> MLSSKYSKRIAWMKTTICDSLQLKDMIVEESFQYEKNKNLLEQFLSGEGLNKIFAYYQVQEQAQNDDIKDTGAQDPVLFFTTGDLEKIQDKAVWFLRITNPADDKKKASQQDGNDNDIIFGEITPNTVPMLNALMESVYSRQIDHIITEKIQFWGVAEEEQVLEFQQHSNKFSSEVREAINLMSPGTEHFKLDYEAISGLSESEKMQHYEMKFNEWINLISSQLNDDSEVRKDEKDAGPATELIYWRSRMQKITNWSEQLKSKDFQIVKASLQRHKNHDNQRPRGDESLSKLMMEYNRLDLLLTDKLNEAKDNVKYLTTLEKFIEPLYNGTPQQIIDTLPALMNAIKMIHTIARFYNTTDKMTGLFIKITNQMIKNCKDRILNKKDNGDNPSLYKMIWEQDPAELIEVLGSCIKLYCEYKKCYNDTKEKVADMPKGKTFDFSDAQIFGKFDTFVRRLQKLIEIFSNIQQFNALAKHNLEGMDVLTNKFKKIIDDFKKKGHNLLDTANNKFDRDWVEFNVEISHLDGELQNFIDNNFNRFRNIEYSLKLLHKFQSTIKRDSLKHNLTSRYNAILHNYATELDTIQRVFQDQKSNPPLVRNMPPEAGKIIWARHLFQKITGPINIFPENVINSTEIRRYYGSYNTLGKQLTIYEMWFYQDWVNKIEQSKAALQATLIVRHDENKKLYVNFDLEIMQLIREAKCLDRQGIEIPESARIILLQEDKFKTYYNELLYALKEYERINSKIKPICKNLLLPHIEDLDLKLRPGMVTLTWTSMNIESYLYYVHQGLKKLEQLIINVNDIIENRIENNLKTVSKVVLVHLPQDTKPLSLDSFVQLQEEYINSKTDFLTSKNVEVERAVDDLLQTIMLYPLDPHVDPVLPEETKRIKRYYFWYFYQALLNSTQNSLNAMKYRVCGKKIPGANTLQNLKPFFQVEVQLNGDKVTLNPSLQEIQKSINRAATAVLRCSKHLYNWDQQNKDSTDKATFYDMIACDKEIVKVILLLTGSIQGTKNKVNEFLSGFTKFEWLCKESIQESIKKFSKNGPTLQNYEDQLKKFSQIEEEIEKIVPTYKIGAMELMTHNICTSLSTWAKEWKLQYSQDLHKRARQLLDSLTEQTKMLSTKLSKPVKDIDSLGYVMETLEQIRKEQAEIDMKFNPVQEMYSLLDNYLPGGITDKDEMDARSLLRRNWDILIQQAEIKGKEYQHKQAIYLKELKQSIKDFTNQVSIFRRDYEKNGPMVEGISPAEAMERLRRFEDEYDVKYQMYKINARGENLFGLQNQKYPELEKTDAEIKNLNKLYNLYDSVIKNIQQFKEKSWQDVSKDDLAKMEEDAGKYGEQCSRLPKDLKEWQAYRDLKNYIDSLREQLPLIISLKKPSIMPRHWEKIKEITNTKLNYENPDQFYIEEIMGAKLLDFREDIEDITESADKQLKIRTGLDEINLYWNDMQFQFGIWGKRDVPCMLNGLIVGTILERLEEDQLQLSTFNSQRHVTPFKAEVENLIRTFSDVNDTLDMWVKVQKLWTSLEPVFTGGDIARQMPLQAKQFQGIDKNWMKIMEKAVETKKVIPCCQNDMLKDFLPDLNRKLEDCQKMLEAYLEGKRKKFPRFYFVSNPTLLKILSQGSEPTSIQEDFEKLFDAITKVTFESAKDKKNPALKQITQIQQVIGRNEENISLTGYYVKCEGNIEDWLKKLEQNMQQTLKDIASAAAQQVFQVGLKEFVSSQASQIALLGLQILWTSKVNEGLERLSRNERNAMDIKRNEIKEHMNILSSMCLEDLNGAVERTKVETLVTIQVHQKDISMDLKCKDVNDFEWQKQTRIAWKTDIDECIISITDWDSPYSYEFLGAKERLCITPLTDRCYITLAQAMSMYYGGAPAGPAGTGKTETVKDLGRTLGVFVVVTNCSDQHRYRDMAKIFKGLVQSGLWGCFDEFNRIDLEVLSVVAMQVESITTARKQHMKKFMFPEEEIEIELIPTVSYFITMNPGYAGRQELPENLKVLFRGVSMMVPDREIIIKVKLASVGYLQIDLLAKKFNVLYRLCEEQLSKQRHYDFGLRNILSVLRTAGNTKRQEIKSDEEMLLMRSLRDMNLSKLVADDIPLFNGLLADIFPKLKEVPKKLYPDVEKKIPEEINAESYLINTPSFQLKIIQLYETCLVRHGFMLVGPTGSGKSTIMKILTEVLTKLGSPHKIVIMNPKAITAEQMYGVKSEISDDWIPGVFSTIWAKSNNRALKHTTWITCDGPVDAIWIENLNTVLDDNKILTLANGERIAMTENCKVVFEVENLNNASPATVSRCGQVYVSPTDLGYEAVIEGWIRNRKASGRAEESDKLGNILRKYLINMRFIELQSKECKEPMMDTSPVISVINILNLLTGCLQYFVQTQRTLSEQEYEKFIVYSMAWAIGGIYEAQDRVRFHELLLAKNAPIPQKGKENETVFDYYVSQDYLDWKICSPEEWVPPQSLQFSQLLLPTLDSFRAEMLLNFILTQPKSHTCSNSALLIGGSGTAKTSSVLLYCNKFDPQKMLFKRTNFSSATSPFMFQSTIEAECDFKVGKEFAPPGNKMMTIFIDDMSMPFVNKWGDQITLELVRQLIETGGFYMLDKTQRGNQRKMKNLQYIGAMNHPGGGRNDIPNRLKRQFFIFNMILPLSIEGIYGPIIKHMFKQKYFSDSTYKVIESLTSATIALWNKVKSTMLPTPAKFHYVFNMRELSRIFKGILTCKKDTINDAPKSMKIKPELFLVGLWRHEAERVLADKLVNNKDKDTVMGYIQEVSLESFSQIENEILEKYSSEKTFLFCDFLRPDVINEDGIIEEEAPKIYEAIDSLTELRKRCNFLLSFYNDRNPSKKMPLVLFDDALKHLLRISRIIRQPRSSGLLVGVGGSGKQSLTRLAGFIGKNLIQQIIVTKTYSDKDLKEDIKKGFDDAGHLGKQVTFLMTDSEVKKEEFLEYINMVLSTGEIPNLLAKDEREVWLGDISQAYCKEKNLGNIDPPQSELWTYFVDRVRDNFHIMLCFSPVGQKFRERARKFPALFNECTIDWFLPWPEEALVSVAETFIKNFDKLDTKEETKQELMKHMGNVHLMVNEICDEYYQKMRRQVYVTPKSFLSYLNSYKTLYIEKYDELDQQEESFKIGLNKIQEATITINQMEISLKEEEIQLNEATEKTNQLLANLDKESKKANQKGEEVAATNKQCEIQAEQISKEKEEAERELEAALPALRRAQEAVDSIESKDIVELKANKKPLDIIKYIMDAVLVFFKARLIPIQIEERVFNKKEGKAVLFLKESYDESGIQTLGDMNFMKKLKEFEKDSINEETIELLEPYLNQSEDWFNDTFATKASKAAAGILKWAFAIYEYHQKSKIVKPKRIQVAIAEGRQAIALKELEKAREDLAQIQAYIKNLKDVYTKQMEEKNELEMKAAKTKKKINTARTLITSLSGEKDRWGKGAQDISDQKRKLVGNVSLSTAFISYCGPFNAEYRNKLAQQRFVVDMKKRGVPVTPGLELTSFLIDDATIGEWNLQGLPKDDLSIQNGIMVTNSARYPLFIDPQGQGQNWIRNKLSASIIPERCITTLSHPKFKDMFLKYCMESGLTLIVENIENEVDPMMDPVLERQIIVKGKTQFVNVAGTEMELSKEFKLFMTCRLANPSFSPELSAKTTIIDFTVTQSGLEQQLLGKVISKEQKALEDSLNQLLADVNQNQKDLQRLDKNLLERLINSQGNLLDDTELMDVLNNTKTQAKEVAAKLIDAEIKTKEINEKREQYRPVAIRGSAIYFTMIEVSLVNWMYNSSLEQFLKLFIESIDLSEKAQLPSNRVKNIISFLTFHVYRYVNRGLFEKDKITFILMMAFKILTTAGTISSGDVSLFLKSGDALDIKSERQKQISYLEDNQWLNILALSKHTFSGQTLPFFKELPDLISRSENQWRNWIDKNDPENFPIPDFAESINQEKEIGSFISLCLVRSLRNDRTLIATQNFISNVLGKEFTDPISYPIEGIWQESSNMDPVLFLLSAGADPTSSIDELAKKKKKFPCEKVSMGEGQERVARQVIMKGFVEGGWVILQNCHLGLKFMEEIETLVSPINQIHEDFRLWITCEQHPKFPLGLLQKTLKVTNEPPKGLKAGLYKTFTTIITQEFIDKVDHSNWRSLIFTICFLHSIVIERKKFGPLGWCVPYEYNYSDLEASLLYIEKYLTNLMSTPQPNSHNLPISMNVVRYMICEVQYGGRITDDLDRELFITYGETYLKDGIFGNDYFFYDIMVDGSGQKFKYRIPQNPSAELIKYQEYIAKVPTVDNPEVFGLHSNADLTFRLKESKEMINTVMETRPKDSSVGGGKTREEIVQDKAKDMLKNLPPDYNDVEVRELVSKLGGPNPKTSTERGMTVPLNIFLYQEVTRMQRVIGLVRKTLQDTILAIDGQIIMTPEILEAINAIYDAKVPNSWLYDPSGAEISWLLPNLGSWSTSLSDRNKQLNDWLRSGQRPILFWLTGFFNPQGFLTGMKQEVTRNHKKKDGKGGEAWSLDDVVYSTTVKEREKEKDIEQPPAEGVYIKGLYLEGCKWSKNGLDDSDPKKIFADLPILHVSAINKKKTNEQDRMSNTYLCPVYKYPKRTDKYLIFRVGLPCEGSNNPSHWKLRGVALLCSTE;> MGDHSQKDSPEDFIINRLSQALGIQKEKIKKSLETQQDDKGEVTNKDEFQGFIQQDNSTNILWVSGQSEKCTFYYGQLPPIDKFKKKGIAVIKLGLHKLTNENVAKDVVVVEITNNLLEHLNSVFNEIMSPVMQNPLNQQGWTDLVAKDLMEKFNNYVAQVYVLLGQIKGKTMLPLPSHKLTSSDTTPDKDKAHVFEGSIITWTKQIKNVLKLEPEQLLKYGNDPGPLAEIEFWQNKRDNLNLIDSQLKSVEVQNILHFLDNNKSTYTTPFTKLQAEVKKARLEANENYRYLFTLKDLFSKLQESQPSDFPTLYELFIPIMHTILLIYNKSKTYNQPPRLVVLIREICNAIISNAQAFVDKDTIFSLIDSKETTEACDKLQVTLDVCSKFKDAYFEYKAKAGGNWKLTSNALFVRLDSFLERCQDILHLTNTIVQFNKLEKIELGGTKGKTLTESIAQIFKEFEEAVQAFTSVSYDIMNIAEKKFDDDFYEFRSKIKELERRLASVITQGFDDYDTIYGRFKLLDNFEGLLTRPIIADELEKKHIVLLEMYKQDLKQVQSIFLEGKQFVDSMHENAPLFLNMPPIAGALTWCKSLRDRIQEPIEKLAQLGQGITEREEYKDVQKLYTSITKSIKDYEDQKILSWEKEVEDSSQDKLKQTLLCKDENDLIKVNFDPSLVRLLKEVKYFLLLRLEVPTTAKDIYTKAETYRTQIVALDMIVDNYNHIKTCLLPVEEPLVKKKIQDMEEEVKPGIEEIRWKSTNIDQFISKSKSIVDQLFETVNKMKDSLQKIHKSLANFNVKIIERKNRPMSPDDYDQFLKAIFSNKLTIVKDNGNQIQKLVKEVLDAVKADKKQNSWKNYNDYVNVIVIEGISTAIQTALLHLNEQINPVFIKRNDISPLFDIRLELGQSGIQFDPEIGESSNQLTVRNTIRNWINDFFNIAGTIQRLDTTMPGDFLQEIRSFFEIKQCLAMITQNLEWIENECNQFRARFDTYSYLWTEDEQISFNRFLDENEPKDEDGKGGDDDEGENTEKQNPLLKGCRAKIPNLDLFDEKITHLKAIQQEISRIKTPEDISWLRINLQPMKTALDARVTRWIRVYTDFLVNQFRTTQKNLLDFIEKTKDGIKKNPADHENLHDKKLLMSVMKVISDVKDVEPRREGIITRMKEMVTKLKKHNVPITEKGTDDPLQQIDNANSNFIEIYGRVFKVKADIIPLQAEETQNIKRDLDIFMKEVESFRKEFMQKLPFDYTESMGYENINNAYDTIMVYYHKLTAIEGRALEYNNLEKLFELQKSNYKQLKDCMNDLKNLKTMWDAIALIHFQYNDWKTKPWRQIKADILLDTNKTLGTQIKNLPKEIRNFKGYNVIVEKVKNMGTVLPLVSALHSEFMEDRHWSQLKQITGTVFDHNSLSFYFEDILALNLYKYENTVNEIVDVAQKEAKIEKKLKNIEQWWSKQVFEFTEYKETKTFASLDNMMEVLDQHSLDLMGMKSQGKYVEFFYDRVEDWREKLGRVDVVVNEWLKVQKNWKILYNIFLLSEDIRMQLPEDTKVFEGVDKEFKDMMSEVSANPSVVEACTIERRDVLVGWSQAIKKCEKALNDYLEQKKKSFPRFYFLSNQSLLTILSNGQNAPKVCEYLGDCFDGLKTLTFEPPANPAETSKVGIGMISKDDEKVPFSSKFICEGAVEHWLLNLEFRMRETLQEILEGAKNTADLWDSGDKPREEWVEGYNAQIALLTTTIVWTEDVGRAFEDLAGGSETAMKECQKLIEVRLENLIKKVRGDLHILERWKIINIITIDVHSRDVVEKFVIQKVSEAESFAWLSQLKFYWENKPDSDMHLRQTLRFPWEKDKNKNKCIIRIVDWFRFYSYEYIGNAIRLVITPLTDRCYITLTQALNLTMGGAPAGPAGTGKTETTKDLGRAIGIPVMVFNCSDQMNKDSMAQIFMGLSQSGAWGCFDEFNRISIEVLSVVSTQVKCVLDALKEKKTKFSFVEEGEIQLQDTVGFFITMNPGYAGRTELPENLKALFRSCAMVVPDLALICENMLMSEGFTMARVLSRKFVSLYMLSRELLSKQKHYDWGLRAVKSVLRQAGKLKRGDPDMPEDPLLMRALRDFNMPKIVTDDKVIFRRLIGDLFPKLDPPTKQNPELKKIVQDTTKKDMGLVAEELFVTKVVQLAEILEVRHCCFVIGPPGSGKTCVWKTLIKSYINSGEDAEYDTLNPKAVTSDELFGAYTKTKEWKNGVIAVIMKNQVKNEEKYKATHMHKWSVLDGDIDPEWIESLNTVMDDNKVLTLVSNDRIFLTPQMRLIFEISNLRNATPATVSRAGVLFINETDIGWMPYMNSWLERSQINILKQQKEMANMPEYPVIDDVAKSVFYRCFQSYFEQNIDVHDKNRVRHICPMVDIAMIQTICTILDALLIQHLPKLKQMKEEDEKQALEAFFIFAGLWAIGGPVGGGQDDSKDMKEFNTVWKGAAKVKFPEQGLCYDYYYDINENKWNTWKVEDYLPNDQPLFSKIYVATIHTTRLRYMIDIHLQRRKPILFIGSAGTGKTAVVRDYLNSTRPEQVSHKTINFSSFTDSLALQKNIESMVEKKNGRNYGSATNKVLICFIDDFNMPYVDKYGTQSPIQLLRLILDYGSIFNREQLEERKFLQDLLFFGCLNQKSGSFTVDLRLQRNFSVFSMYTPSSDVIKTIFGSILNAHLSTIDDKAQKMAFKLVEATYFTFDKILKNTTAFAPSAKRFHYQFNFRELARVCEGICRTTPGQYSGGDQGKLVRLWAHEMKRTFEDRFIANEHVEFFRRYLTEAISKCIGEFPETENPIAEPLIFTGFVAAHQGLDQQYTQCTIPVLKRVLDDKLEEYNEVKAQMNLVLFQQAMEHVSRICRILDMPGNNALLVGVGGSGKQSLCRLSTFINGFEIDQLVVTASFTINDLRNNLQEIYKKIAKPNSIARVFMITDSQIKEEQFLIPINDMLNSGWIFDLFPKEDMDSLVSGVRNEAKGEGVDVNNLTALTSYFLDKIRKNLKVVLCFSPVGDTMRIRSRKFPGIINNTSIDWFHPWPHEALIDVAFRFLEEIEFPTEEIRQSISLNMAKVHSSIDTANEKFLKLERRYNYTTPKSFLELIDFYKKLLTEKRETIQRQIQRYEMGLNILAETQNKVQGLQEELKVKMVEVNKQREETDILIEKVGKESALAEEEQTIANAEEEKTNVAAAEAEKISKEATEALAEALPALRSAEAAVDCLKKPHVTEMKNLGSPPAGVIVTARVVLILFNQGITLNDPDEKVWKKAVTFMNNPQAFIDKVKSFDGENIEPNIIEQSNKIIQDPSKKFNEKDMAGQSYAASKLCAWAVNIVTFNKIFKQVKPLQDAQKQANEILEEKKKELAIVKQRVAELNARVNSLKRQLEEAEARKMIVEQDAARCQSRLSAAENLVNGLAGENKRWTQNVKFLKENIKSMIGDSLLASAFVSYIGAFSAKLRLELWKNTWLPDIIEKGIPITEGIEPLKILTTEAIKSKWKNEGLPADPMSLENAAIITACARWPLIIDPQLQGSTWIRGKQGENLTTISLSQPKWLGALTSSISSGRAVLIEGIQQEIDATLDPLLQRAVKKNGNQLQLEIGGDPIDYDPNFKLFLMTKLINPHFRPEIAAQCTIINFIVTESGLEEQFIAMVVNIEKNELEMAKQDLVKKQNEYAVTLDKLESDLLQSLSEADPATILDNTELIQNLDKTKKTTIEITEQQQKAKVTEAEINIQREHYRVVAAEGSMLYFLVISLSVMDHMYQYSLESFITFFFKAINRTTVRDENRIPTLILNIRQTIYQWISRGLFEKHKLIFLTLIVFRLMQKKIIDVAYEVAEMDFLIKCPARPGVENTLDWLPNISWDQIQGLINLEEFRNFAHQLEKEAPNRFKDWYNELQPEDQKLPLDWKRLDSMPFKKLLVLRCLRPDRMTISLNNFIRAVLPQGDAFVEMDQKLAFSEILESVINEDSESTIPIFFILSPGSDPVKEVEKIAKKKRIEPGKNFFNIALGQGQDEIARRRIEEGNKEGHWVMLQNIHLMPTWLIELEKILDSYSGEAGGGNSEFRLFLSAEPSTGIPIGILDRSIKLTNEPPAGLKANMKRAWTYFSKEEIEDKDPKIKSILFALCFFHSTLIERRRFGPKGWNMSYPFNMGDLRDSYLVMNRYMEQNQGGKVPFNDLIYIFGEIMYGGHIVDDWDRRLCNSYLFNTMHEQLFDELELFPYIEGKGLSFKVPGQNPYEKYIEHIETSLKQETPLAYGLHPNAEIGFRTDQCKTLFNTLLELMPKEQSRDEKSSDIKSSNEMASDLIKQLLEDSELKNKIFNMEEIKNKIDAENKGPYQNVFLQEIEYMNALLSEIVKDLEEIGQGLSGLLTVSENMEMIIESIALSRVPASWQKLAYPSKRGLQSWLANLFQRIEQLNIFRDDPYSIPRVVMISRFFNPQSFLTAIMQVISRAKAYELNKLYIQTEITKRSIEEIEGAAKEGAYVYGFILEGARWDYQLGQLEESKPKEMFSVLPVTYCKAIPLPPEGKEDKSLYQCPVYKTEDRGNTYVFTAQLKTRFPPRKWILAGVAIIMDVEGVSDEVKKDKK;> MPQPLVWTQLKQTGTTQPTARSGHTIITVGKTHIMFGGLDNDKNNYKDGKIAPNNQVFTLKLTQNNCEWRQIACQGDVPLPRCYHASCAISADKMLVFGGSYTSNLRFNDTYILKTTSYQWSKPANQISGGEPKNAESKIGAPQPRYGHSATFFEGKVYIFGGHGGINYQRLAFNDLYVLETENFEWTRLEPKGNPPDPRGGHSAAMMANKPQLMIFGGWSFTSQYSNIMIYDIEKDEWVDPEIAHEIPKWNLSGIMAPSIPSWKYFIFGGSVGSFEEGGNRTNSRFVDDSFVLDIDTLSWSSINLEADETSKAVCKPRPRESASIFYDSGESRAIVFGGWANNWLNDLWALNVSTITGPPYAIFSIKPALGPLTGKTKVLIEGDGFKDTQNISVKFSGGKLEKEVNGTFVNEKEISCETPTFDYPRSVEVTVCMNKGDYTITKSAFTYYLNTKADKTIAYGPGLLTENLIGVQTTIVIQARNKNDQNRESGSDEFVVTIRNPAKIKKEEEVKEGDKANTKNTIKEDEEEEGEDEEENKKKKEAEKAAAEKAAAEKAAEEEQGEAVDPSLVPFNIVDNDDGSYFIQFTSEEEAVLEIDIKFKDENNELHSIRGNPFRCGFVKGSKPNNNDLTGSAVMNYISKQLKDIQEFIENTKENIEIRNKNIRENVSELINVMINLEKVRVKNDDDVLTLDTVEEMLNFLKKKDFGKDSDIKKCKKLQEEWKNLAKMAQAVKKDIQNPVKTESDKTKENIKKFEEITLKEYANSLKKESFFIYKTGVSESFKRIG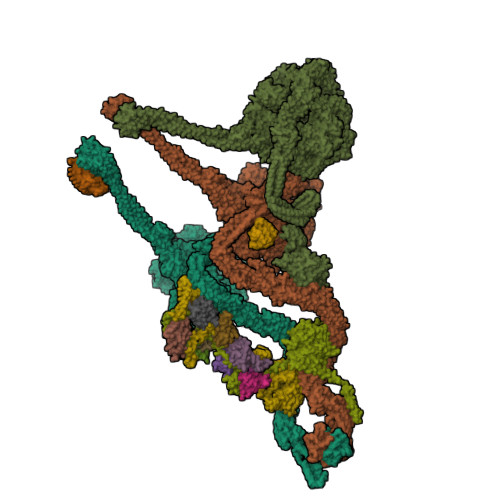EVKQKVDEFEVQLNQYEDFARMFEFPDAVIGSKKLMEQIRTDVSSVEKLWVRIEISEKTMDEYKKMKWGSINSMDMEDEIKKLRKALTDLRGIDKRSNAFIGITEELKKWATFLPLLGELKDPSMNSEDGRHWKKLKDLVKKEFDVSQELMLEIIWDLKLFDYKDGIEEITDQAKQELKMEKALKKIIDFWRDIEFELVQHKNTDIHTLKMSEENFETLEDHQLQINNMLLSKYVAYFEKEVEKWKYDLGSVYDVVQLLLEVQKTWSFLENLFIQSEEVKRELPNESAQFVGIDKDMKEIMQKGCDIKNCLKFCTIEGMLKRLENIQAQLKVCEKALNEFLDSKRRAFPRFYFVSVNDLLDILSNGNSPAKINRHMSKIFQAIDNLQLKEDSSGGRPTALKMISCVGTEEVDFSSPRLLQGKVESYLKDVIDTMIGTLKSVANSSFKNFQSMTRKEWLKSDPSQITLLVNNIIWSKAVEDCFLKLQSGDINAMKLFLDESIKQLTELIGMVQGDLSKPLRQKIMCLITIDTHSRDVVHRLINEHVRKAEEFQWQSQLKFYWVDNDAKIKIADARFVYNYEYLGNGPRLVITPLTDRIYVTATQALHLKMGCAPAGPAGTGKTETTKDLANALAKACYVFNCSSEMNYESMGNIYKGLASSGCWGCFDEFNRLLPEVLSVCSVQFKAVTDAIKQNVERFIIEGDEISLDPTCGVFITMNPGYLGRAELPEGLKALFRPITVVVPDLELICENMLMAEGFIEAKILAKKFVTLYMLCRDLLSKQLHYDWGLRAIKSVLVVAGGFKRSEPEIAEQALLMRALRDFNIPKIAFQDLYVFHGLLGDLFPGINIKPKKDLDFEKIITDVCIENKLDPDPEFVLKVVQLSELLAIRHCVFVMGPPGAGKSTTWKILAKAQDKTNKKTTLIDIDPKVVSTKDFYGYNLPSKEWKDGLFSKMLRSLAEQPDTNPKWICLDGDLDANWIESMNSVMDDNKILTLANNERIPLKPHMRALFEIRDLRFATPATVSRAGILYISDEVGYQWRSYVKSWIKQEFSQDQEMSKNLDTLFGKYVPDTLDHIKKHCRFLVPVSPISQVISICKSLQTLLKGDVKNLEYLFVYALIWAIGGALAEKDSIDYRKDFSTWWKGAWKTAVKFPSKGTIFDYYVDQSGDSSKFVEWSKRLENKEFDPQVETMGNITVNTIETLATTEFIKSYLMVKHPSLLIGNSGCGKTQLAKGILKEIVQAKPENYAYQLINFNYYTDSTYLQGQIEQTLEKKAGRQYGPPGKVQLIYFIDDLNMPQLDAYDTQTAIALLRQLADYGHFYDVSKLALKDIINTQVLAAMNPSAGSFFVNPRYQRHFWTISIPFPDNESLSLIYITFLNGHLKRFKSTIQEYSNIIVRASLMLHQAVTQNFRKTAINFHYEFNLRHMSNVFQGLLLSDPNKFTEPDKLIKLWIHECERTYGDRLVSTDNLKTYKENIFDIVKKSFSKFNFSRYFGNNPENLIYCNFIAGINSDRFYDQMPNNEMEKHISEALKEYNDNNAFMGLVLFEDAMKHVCRICRIVLPSSGHALLVGVGGSGKQSLSKLASFIMGYTTFSITISATYSMVDLRNDLQQLYFKCGPKEEGILFLFTEGQITNERFLVYINDLLSSGEIAELYTLDEKEAMINQVRAKVKGEGKPDTRENCWNWFIDQVKKNLHMAICFSPVGDMRRRARQFPALVNCTVIDWFQPWPYEALFNVAKSFLEPVDLGDDKVREAVVKFMPFSFTLVNDLGLKLLEQERRYAYTTPKSFLELISLFTNMLAQKRESLERNKERYETGLVKLKETAEQVAIIEVEVKEKQVEAEAKKKEADAFAEVVGREKDKVEKENSKATIEADKCGLIKQNVEAQKSSTQQDLDAAQPLVEQAKSALNSISKKDFQQAKSFASPPAGVPEVFAATIYLLAGYFNEAIEIDKNKKPKDVSWKSSLKLMKSPEEFMEKLLNFKDVVDANQVPAANVNIVKNQYLNMPSFTPEQMASKSAAAKGICSWVVNIVKYYDVIQDVEPKRKALKEATEQLEEATVKLNEVEEVVRKLNEELNKLKAENDKAIAERNAAISEAERCARRLNLAQRLVTALSSENERWGKSIIQLEDQLKLMVGDVLVASSFVSYSGPFNKKFRNIMINQNFMKFMKEHTIPMSPDPNPIKILTDESTIALWNKQKLPSDSVSIENGTILTNSARYPLMIDPQLQGITWIREKEKANNLKILRLGSKNINRDLELSIENGYSAIIENMNERIDAILMPIIARSFIKRGKNKIIKFAGKDLILHPNFKLFLHTKLSNPHYPPEIQAEAALINFTVTEAGLGDQLLSLVVARERPDLAKMKIELITQQNDFKIKLKDLEDELLYKLANAKGDILDDIELIENLEYSKKLSVEIAEKVAAAKITEAKINETSENYRPAASRGALFYFLLSDLSKVHSFYKYSLESFIVVINRAIDAISENKIYGKTTMVPYGDETYASNQHEKEEEEEEEEHQQAQQQQNQEEQQEQKDEENKGPVEEEQPEGENKGPVEEEGAEGQNEGPVEEENAENQEGEGEEEGEKQQKAKDSDEPMSPRSLKKRVDELIESLTYTAYQTTRRGLFESHKLIVAAMLCLRVLLRSEELNSDEVDHLIIGKVDVNPTPMPDALKSFLNDNIWAACKALETIHQFQGFCQSLETDVLQWKKWYSEEKAETADLPKAFKELSKFHRLLLLRALRPDRLPSALSQFVHDKMGERYIEQPPFNIFETFQETSKTVPIFFVLFPGVDPTPDVERVAATFDVSANNGRFINISMGQGQEDRAKKALFDCAQKGHWIMLQNVHLMQSWLYGLNGLEGFLESVFASPKTHPNFRVFISSEPPNVLLPLMQIIPESILQGSLKIANEAPQYLKANLRRAYNKFDQEFLDKCDKKPTEFKSCLFALCFFHSLMLGRKKFGTQGWSRVYNFNDGDLTICADVLYNYLSKYDQVPWDDLRYIFGEIMYGGHITDDWDRRTNRTYLKVLIRSELLQQNFNLAPQFKSPDPSKFDYEAYRKYIEEKLPIESPQMFGMHPNAEIGYLTQTCDQVFNTILEVQGGSSGGGASKKDDGVMVTLTDFKTRCPHDFNMLLIEEKVKEKTPYIVVCLQECERMNGLLKEIKTSLEDLRLGLTGALNMTDAMESLQQSLSFNKVPDTWEKKAYFSKKPLSSWFADLIERNIQLQEWCKELVTPTSLCISYLFNPMSYLTAIMQFTARAQGLPLDGITIQTNVTAMKGPEDVVNPAENGAYIHGLFLEGAAWEIGGQGQDGYLIEQKPKELHPKMPVINAVAVPLDKKKKNGQYDCPTYVTSARGQTFVFTANLNMESDDSDPNKWILSGTCMLMSDD;> MPPKQTKVVASRKTVMPISRAGRAQIRRKDSNTQNNMNDQGMEDEEIDQQREGMKNQYEQLTAQELNEDMPSKMLEPKNPQAPKNITVYDYYTRKFKTDELVDQMIVHFSMDGDYIWKESNEYKTQEEIRDTKKALIKEAMRKQESEEPGANHDEEAIKQTLRNKFNYNTRECQTINPSIRERGVSTEPPPSDTICGNITQWEIFDAYYAEIMKDHQIENKKKKEVDQDKKQDQSMYSTSFKRCCKIMERMVVQNDQEDKYHDYRYYWSQGDNLEAGKNEGHLLPIWRFSNEKQRKKNVTSICWNPLYPDLFAVSLGSYDFTKQRMGLICLYSLKNTTHPEYAFNCEAGVMCLDFHPKSAALLAVGLYDGTVLVYDIRNKHKKPIYQSTVRNQKHTDPVWQVKWNPDTSKNYNFYSISSDGRVMNWILMKNKLEPEEVILLRLVGKNEEESTLIGLACGLCFDFNKFEPHIFLVGTEEGKIHKCSRAYSGQYQETYNGHLLAVYKVKWNNFHPRTFISASADWTVRIWDSKYTSQIICFDLSMMVVDAVWAPYSSTVFACATMDKVQVYDLNVDKLNKLAEQKIVKQPKLTNLSFNYKDPILLVGDSHGGVTLVKLSPNLCKSGPEIKQTEDKKAMEEFKNVKIEDYEREKMENLLAVVSKWEREDA;> MAEYFTYSKKRKEFNNPINFQDTETRYGGIQNQVVNINQYVQRNPNFIDLDNIAELSEHSVNTERVKTGDRGMSHKEGGWPGNVDPNEAQETGRFKKRIEKDTSFPQAVKDLKEGVEKCIYQNNQIDLLEEYFEGETSEHVVENLSSKTLMLFKDEKEICKRSVSEISWHPEGPTKVAVSYAIMRFQQMPEKMPTQAYVWDLLNPNSPEIKLMSPSAVTNISYNQKIPDQIGGGCYNGLLAVWDGRKGENPIMISPVENSHYEPVTHFHWLMSKTGSECVTTSTDGKVMWWDTRKFEAGPVEKLNIIEGLGENEEIIGGTALEYNVEAGPSKFLIGTESGSILTANKKLKKPVEITTRYGLDQGRHLGPVYSINRSNQNPKYFLSVGDWSCKIWVEDLKTPIIRTKYHGSYLSDGCWSPTRSGAFFLVRRDGWMDVWDYYYRQNEIAFSHKVSDSPLTCIKINQTGGAYHNSGKLCAIGDQDGTVTILELCDSLYTMQPKEKDIINEMFEREYRKEKNLETIKKQQELAKRQVQKDMGSQKEKWEKKKLEMIETAEASFHENLAKNPVNEEEFNELDSPSEKRKKTNQNQGREQEEQSREEQEASGNFNQQQQQQQEEEQQQEGEQQHHQNQEHQNGQGHENGQEEGEENGEEGNQQENEGQEENEQQQE;> MAQDINADDQLKQLSALEGANGYVIFNESGIPLKRHEKSISHEKAVHIAALVSDLWNVSKKVIQRDLKTPENDIEVIRLRTKHSYEYIITQSGDFTMLAIQLCGKAIEEAKKAAAAAAAAAVVQEENKEKEKK;> MIYKTSKEIQKSDQRIIQQRVENSIINNQIYQKSLKRKTSKRKVRHQANKKNFQKEMSEVEDTLNRIKTHKTVLGYLIVNSEGGVVRGAFKDEEESKNIANSIPLLTKKARSVVRDLDPTNDLVFLRIQTKLNEIMVAPDDEFSLIVIQTKGEKRDEND;> MSHLDKVQPVIKNSDMSVEMQKEVEEVAKKAIDYCNTDKEIATFIKDDFRSRYHGTWHCIVGRNFGSFVTFERSYYIYLYVGQLAILLFKTG;> MEQEKAVTDMDINELRKLMIGKAIINSSDMQGDLLQEAQDVIQSGIENNSAPVLNIEAACKYIKENLDKKFGPTWQCIIGEGYAYDVTVQNNTLLFMFYNGNLAVLIFKS;> MASNQQQKEDPKEQQQQYKTFMGARVLWPPECADDILEGAIRETQDALKKFEIAREGQKIAEHLKKYMDDHFDPYWHVFFGKNFGCQAVHNKNRFIYFYIEKTAFLMYQTQ;> MGDHANEQIIDMPENSEMKSMKNDAFSQAKFAVENYKFENKISSHIKKFFDEKYGPNWHCVVGKHFNAYVSYDSKNFIFFYEGQLAILLYRKG;> MSDSDSDEGRVVEEPLPPHIIRFNDMAQHLLKKVIRQADVLIKENPQGLEKDIALNLVKFVKSQPEFKIGDGEWQCIIGKNFGCSLTFDANVLAFFDLLPSRKSILLFKSG;> MNHEPEVKATDMEEDMIKRVKEIAINAVKEYKQEKQIAHYIKYEFDKIDGYGWNCIVGRNFGSHIIHQTKKYIFFKINELCLLLWKA;> MGDTDKEYISEEVQKAIDDSVKQVFGIKDDSSQVTITYNKDKVNLWTQQIIDYTIRGLNKLGKHFKYCVTAILQQTNHAGISVQITAYQDTNTDGSLIQCYEINDIYAIVSVFAMAV;> MKGTYLYLNIYKRKREASLITLNYIKNRFYPSKIQKIIKELFEDRLKGVEYDPNNANQLSERLVLELREKIKRGKVPRYKIGVQVVFGEIKGQGLRIASKCLWDVQNDNYASYTYTSEKVYCTGIVFGCYFE;> MSKKQKKEITTTVTSEDHFMTFYNENNKKLIVVDVYPGWSGPCTAMYPTYNQLMISIDDFEKRIDILLLDQDKLVTYKNDKFHATCQPKFLFISEGKIIDEVLGTNIPVFIEKVNKYIPLSY;> MSKGTTCQKAIVNWEAANPGKNPSEAEEIKLIFQIPPIEKMDGPVLNTLTKCKKLSLSSNSIDKMISLNMLRNLEILSLSRNVIKKISGLEDIGGTLRQLWLSYNFIEKLDGLNNCSVLQTLYIGNNRIKNWEELDKLKDLPELENVLFYGNPIYEQVKEDPKLIVLKKLPTLKNVDGYIIDDSVLEKVKQIADIPISAKQL> MAAILALASATIQAADVTITVNGKVVAKPCTVSTTNATVDLGDLYSFSLMSAGAASAWHDVALELTNCPVGTSRVTASFSGAADSTGYYKNQGTAQNIQLELQDDSGNTLNTGA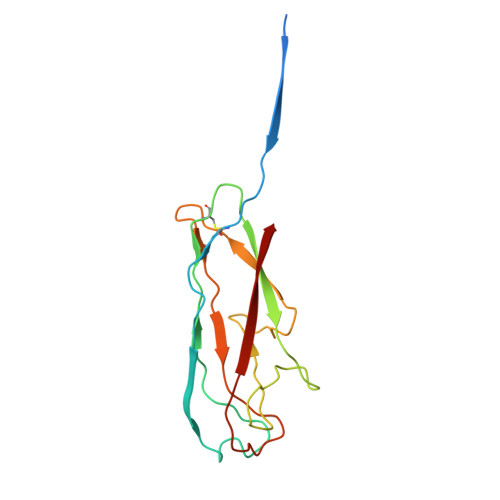TKTVQVDDSSQSAHFPLQVRALTVNGGATQGTIQAVISITYTYS> MGSSHHHHHHSSGPQQGLVRGHMASAADYPIFSQRFTADPAAVVYNGRLYIYCSHDSDATPGQSTYNIPDITCISTDDLKNWTDHGEVFNAKRD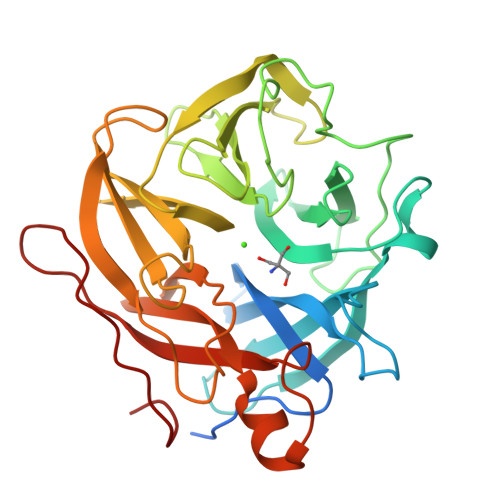SRWASVSWAPSIVYRNNKFYLYYGNGGNGIGVAVSDSPTGPFKDPLPGPLVSWNTPGVQPAQNMWLFDPGVFVDDDGQAYMYFGGNGQNNIRVIKLGNDMISTVGSAMTMSAPRFFEAAYMHKYNGKYYFSYASDFSQGASKIEYMMSDKPTTGFQYKGVILPQPPDNYSNNNHHAIVEYKGNWYVVYHNRTVAKQRGLDPVYQRNVCIDQMFYNADGTIKQVVPTVDGLKQ>[2x]MVLYFIGLGLYDERDITVKGLEIAKKCDYVFAEFYTSLMAGTTLGRIQKLIGKEIRVLSREDVELNFENIVLPLAKENDVAFLTPGDPLVATTHAELRIRAKRAGVESYVIHAPSIYSAVGITGLHIYKFGKSATVAYPEGNWFPTSYYDVIKENAERGLHTLLFLDIKAEKRMYMT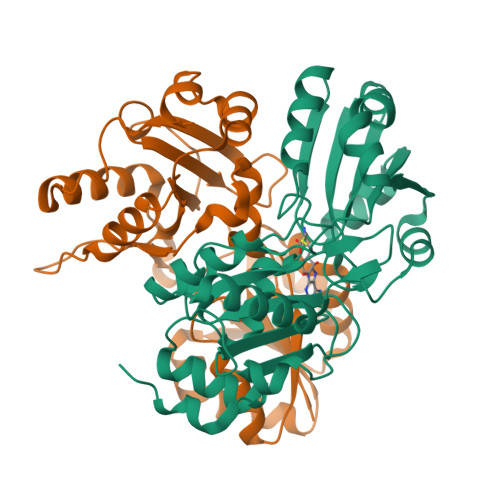ANEAMELLLKVEDMKKGGVMTDDTLVVVLARAGSLNPTIRAGYVKDLIREDFGDPPHILIVPGKLHIVEAEYLVEIAGAPREILRVNV> MSSNRVLDLFKPFESFLPEVIAP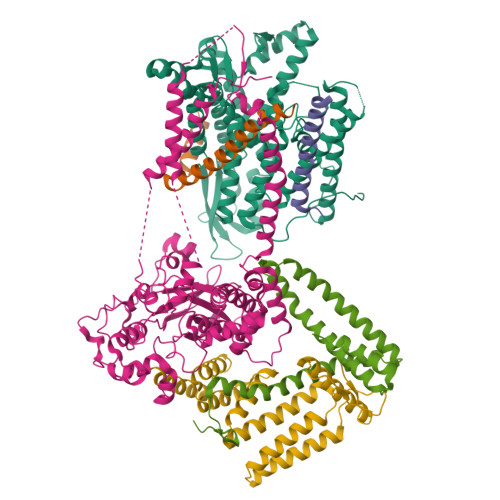ERKVPYNQKLIWTGVSLLIFLILGQIPLYGIVSSETSDPLYWLRAMLASNRGTLLELGVSPIITSSLIFQFLQGTQLLQIRPESKQDRELFQIAQKVCAIILILGQALVVVMTGNYGAPSDLGLPICLLLIFQLMFASLIVMLLDELLSKGYGLGSGISLFIATNIAEQIFWRAFAPTTVNSGRGKEFEGAVIAFFHLLAVRKDKKRALVEAFYRTNLPNMFQVLMTVAIFLFVLYLQGFRYELPIRSTKVRGQIGIYPIKLFYTSNTPIILQSALTSNIFLISQILFQKYPTNPLIRLIGVWGIRPGTQGPQMALSGLAYYIQPLMSLSEALLDPIKTIVYITFVLGSCAVFSKTWIEISGTSPRDIAKQFKDQGMVINGKRETSIYRELKKIIPTAAAFGGATIGALSVGSDLLGTLGSGASILLATTTIYGYYEAAAKEGGFTKNLVPGFSDLM;> MSSPTPPGGQRTLQKRKQGSSQKVAASAPKKNTNSNNSILKIYSDEATGLRVDPLVVLFLAVGFIFSVVALHVISKVAGKLF;> MARASEKGEEKKQSNNQVEKLVEAPVEFVREGTQFLAKCKKPDLKEYTKIVKAVGIGFIAVGIIGYAIKLIHIPIRYVIV;> GGSGGSGGSGGSGGSPTNYEYDEASETWPSFILTGLLMVVGPMTLLQIYQIFFGANAEDGNSGKSKEFNEEVFKNLNEEYTSDEIKQFRRKFDKNSNKKSKIWSRRNIIIIVGWILVAILLQRINSNDAIKDAATKLFDPYEILGISTSASDRDIKSAYRKLSVKFHPDKLAKGLTPDEKSVMEETYVQITKAYESLTDELVRQNYLKYGHPDGPQSTSHGIALPRFLVDGSASPLLVVCYVALLGLILPYFVSRWWARTQSYTKKGIHNVTASNFVSNLVNYKPSEIVTTDLILHWLSFAHEFKQFFPDLQPTDFEKLLQDHINRRDSGKLNNAKFRIVAKCHSLLHGLLDIACGFRNLDIALGAINTFKCIVQAVPLTPNCQILQLPNVDKEHFITKTGDIHTLGKLFTLEDAKIGEVLGIKDQAKLNETLRVASHIPNLKIIKADFLVPGRPYISLKVLVRSAKQPLIPTSLIPEENLTEPQDSESQRDPFAMMSKQPLVPYSFAPFFPTKRRGSWCCLVSSQKDGKILQTPIIIEKLSYKNLNDDKDFFDKRIKMDLTKHEKFDINDWEIGTIKIPLGQPAPETVGDFFFRVIVKSTDYFTTDLDITMNMKVRDSPAVEQVEVYSEEDDEYSTDDDETESDDESDASDYTDIDTDTEAEDDESPEGENLYFQ;> MSEFNETKFSNNGTFFETEEPIVETKSISVYTPLIYVFILVVSLVMFASSYRKKQAKKISEQPSIFDENDAHDLYFQIKEMSENEKIHEKVLKAALLNRGAESVRRSLKLKELAPQINLLYKNGSIGEDYWKRFETEVKLIELEFKDTLQEAERLQPGWVQLFVMVCKEICFNQALSRRYQSILKRKEVCIKEWELKINNDGRLVN;> MVTLEYNANSKLITASDAVVALSTETNIDQINVLTTSLIGETNPNFTPQPNEALSKMIKGLFESGMKNLQQKKLNEALKNVSLAIEMAQRKRAPWEAFAIQLPELHFMLRSKIDLCLILGKHLEALQDLDFLLGTGLIQPDVFVRKADCLLKLRQWEEARATCERGLALAPEDMKLRALLIETARNLAEYNGE> SQIPASEQ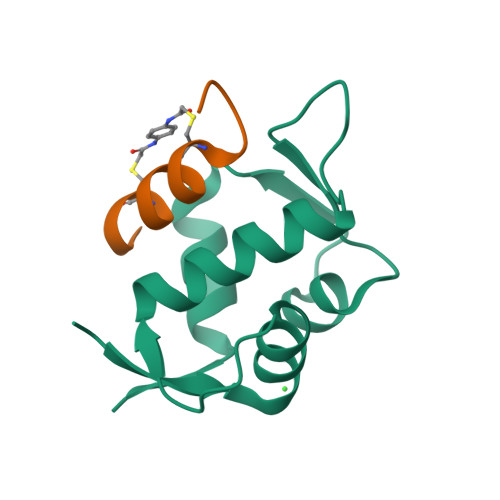ETLVRPKPLLLKLLKSVGAQKDTYTMKEVLFYLGQYIMTKRLYDEKQQHIVYCSNDLLGDLFGVPSFSVKEHRKIYTMIYRNLVVVN;> XDPAHWYCDFAAQVCNFSX> PFKEVSPNSFLLDDSHALSQLLKKSYRWYSPVFSPRNVPRFADVSSITESPETLKAIRDFLVQRYRAMSPAPTHILGFDARGFLFGPMIAVELEIPFVLMRKADKNAGLLIRSEPYEKEYKEAAPEVMTIRY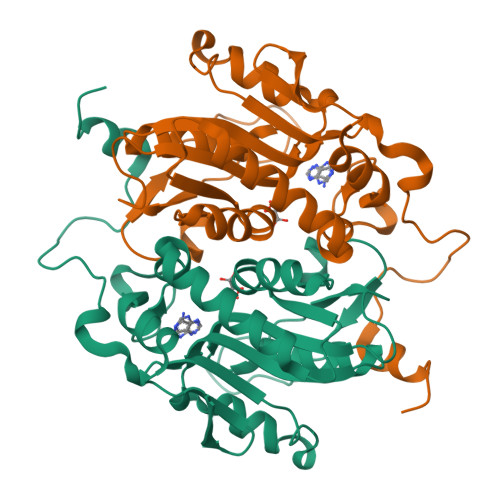GSIGKGSRVVLIDDVLATGGTALSGLQLVEASDAVVVEMVSILSIPFLKAAEKIHSTANSRYKDIKFISLLSDDALTEENCGDSKNYTGPRVLSCGDVLAEHPH>[2x]GSHMNVFNPAQFRAQFPALQDAGVYLDSAATALKPEAVVEATQQFYSLSAGNVHRSQFAEAQRLTARYEAAREKVAQLLNAPDDKTIVWTRGTTE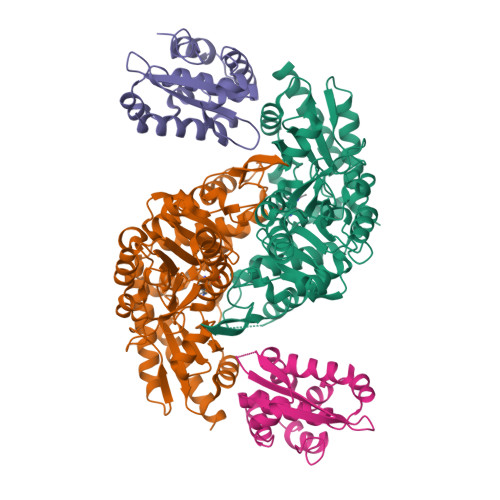SINMVAQCYARPRLQPGDEIIVSVAEHHANLVPWLMVAQQTGAKVVKLPLNAQRLPDVDLLPELITPRSRILALGQMSNVTGGCPDLARAITFAHSAGMVVMVDGAQGAVHFPADVQQLDIDFYAFSGHKLYGPTGIGVLYGKSELLEAMSPWLGGGKMVHEVSFDGFTTQSAPWKLEAGTPNVAGVIGLSAALEWLADYDINQAESWSRSLATLAEDALAKRPGFRSFRCQDSSLLAFDFAGVHHSDMVTLLAEYGIALRAGQHCAQPLLAELGVTGTLRASFAPYNTKSDVDALVNAVDRALELLVD;>[2x]GSHMTNPQFAGHPFGTTVTAETLRNTFAPLTQWEDKYRQLIMLGKQLPALPDELKAQAKEIAGCENRVWLGYTVAENGKMHFFGDSEGRIVRGLLAVLLTAVEGKTAAELQAQSPLALFDELGLRAQLSASRSQGLNALSEAIIAAAKQV>MKNVGFIGWRGMVGSVLMDRMSQENDFENLNPVFFTTSQAGQKAPVFGGKDAGDLKSAFDIEELKKLDIIVTCQGGDYTNEVYPKLKATGWDGYWVDAASALRMKDDAIIVLDPVNQHVISEGLKKGIKTFVGGNCTVSLMLMAIGGLFEKDLVEWISVATYQAASGAGAKNMRELLSQMGLLEQAVSSELKDPASSILDIERKVTAKMRADNFPTDNFGAALGGSLIPWIDKLLPETGQTKEEWKGYAETNKILGLSDNPIPVDGLCVRIGALRCNSQAFTIKLKKDLPLEEIEQIIASHNEWVKVIPNDKEITLRELTPAKVTGTL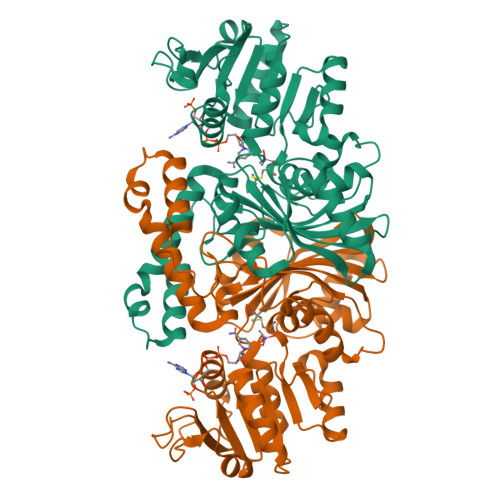SVPVGRLRKLAMGPEYLAAFTVGDQLLWGAAEPVRRILKQLVA[4x]>[2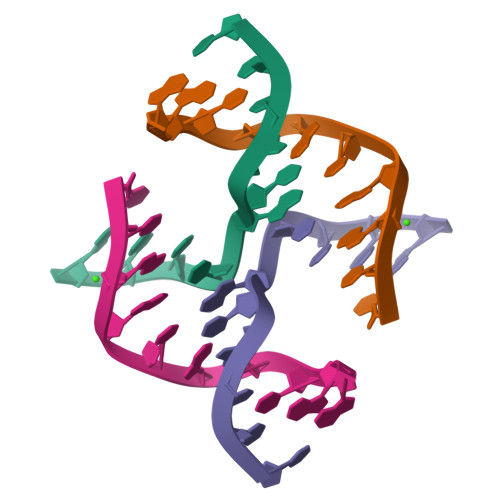x]CCGATATCGG>[3x]GARASVLSGG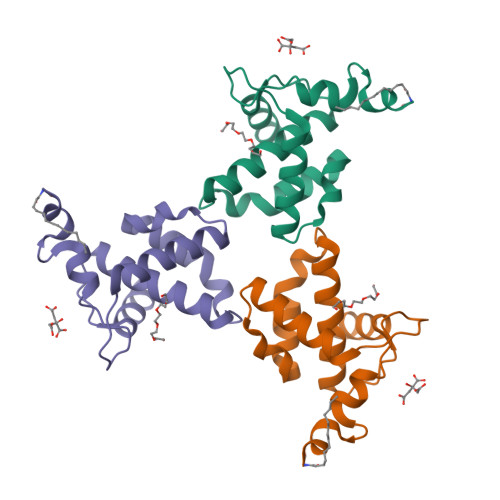ELDKWEKIRLRPGGKKQYKLKHIVWASRELERFAVNPGLLETSEGCRQILGQLQPSLQTGSEELRSLYNTIAVLYCVHQRIDVKDTKEALDKIEEEQNKSK> SMGPTSQRRGSLQLWQFLVALLDDPSNSHFIAWTGRGMEFKLIEPEEVARRWGIQKNRPAMNYDKLSRSLRYYYEKGI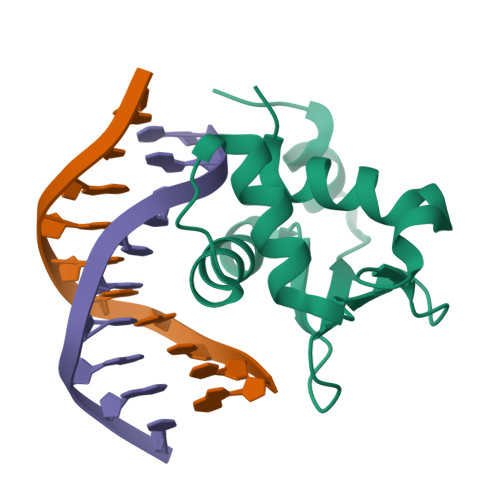MQKVAGERYVYKFVCDPEALFSMAFSDN> HPNSPLDEENLTQENQDRGTHVDLGLASANVDFAFSLYKQLVLKAPDKNVIFSPLSISTALAFLSLGAHNTTLTEILKGLKFNLTETSEAEIHQSFQHLLRTLNQSSDELQLSMGNAMFVKEQLSLLDRFTEDAKRLYGSEAFATDFQDSAAAKKLINDYVKNGTRGKITDLIKDLDSQTMMVLVNYIFFKAKWEMPFDPQDTHQSRFYLSKKKWVMVPMMSLHHLTIPYFRDEELSCTVVELKYTGNASALFILPDQDKMEEVEAMLLPETLKRWRDSLEFREIGELYLPKFSISRDYNLNDILLQLGIEEAFTSKADLSGITGARNLAVSQVVHKAVLDVFEEGTEASAATAVKITLL;> SALVETRTIVRFNRPFLMIIVPTDTQNIFFMSKVTNPKQ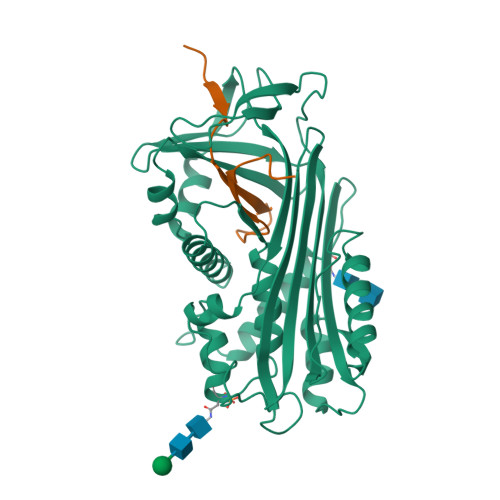A>LNSINTNAGAMIALQNLNGTNSELTTVQQRINTGKKIASAKDNGAIWATAKNQSATAASMNAVKDSLQRGQSTIDVALAAGDTITDLLGKMKEKALAASDTSL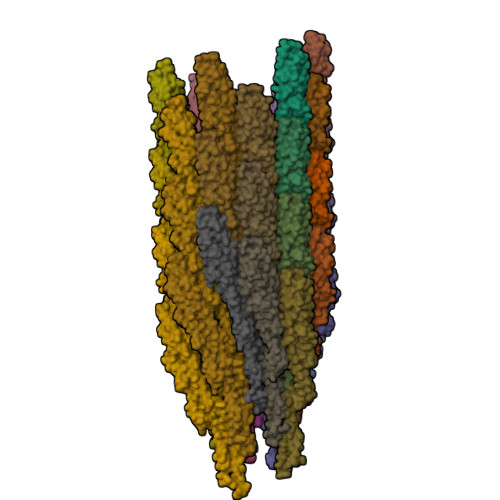NTASFNALKSDFDSLRDQIEKAATNAKFNGVSIADGSTTKLTFLANSDGSGFTVNAKTISLAGIGLTTTSTFTTAAAAKTMIGTIDTALQTATNKLASLGTSSVGLDTHLTFVGKLQDSLDAGVGNLVDADLAKESAKLQSLQTKQQLGVQALSIANQSSSSILSLF[36x]5-FLUORO-2'-DEOXYURIDINE-5'-MONOPHOSPHATE 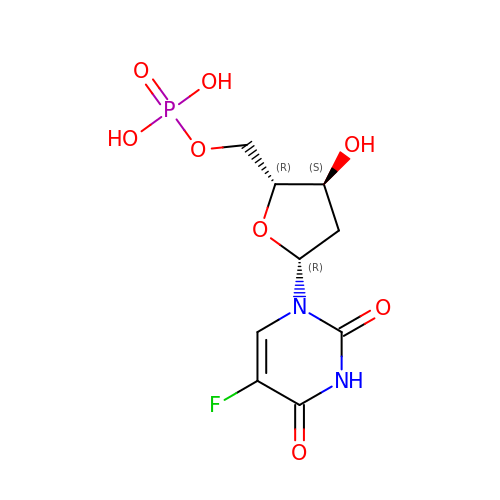| C9 H12 F N2 O8 P | HFEKDTCAMMOLQP-RRKCRQDMSA-N>[3x]MKILVIQGPNLNMLGHRDPRLYGMVTLDQIHEIMQTFVKQGNLDVELEFFQTNFEGEII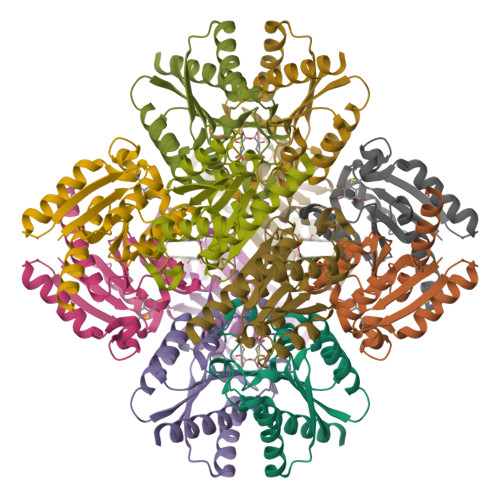DKIQESVGSDYEGIIINPGAFSHTSIAIADAIMLAGKPVIEVHLTNIQAREEFRKNSYTGAACGGVIMGFGPLGYNMALMAMVNILAEMKAFQEAQKNNPNNPINNQK>CGATCG[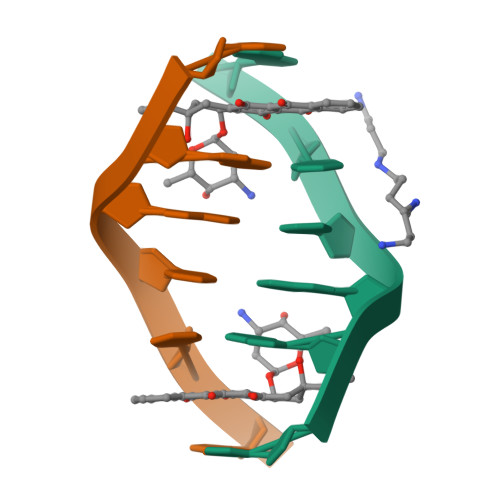4x]>GSHMSDWDPVVKEWLVDTGYCCAGGIANAEDGVVFAAAADDDDGWSKLYKDDHEEDTIGEDGNACGKVSINEASTIKAAVDDGSAPNGVWIGGQKYKVVRPEKGFEYNDCTFDITMCARSKGGAHLI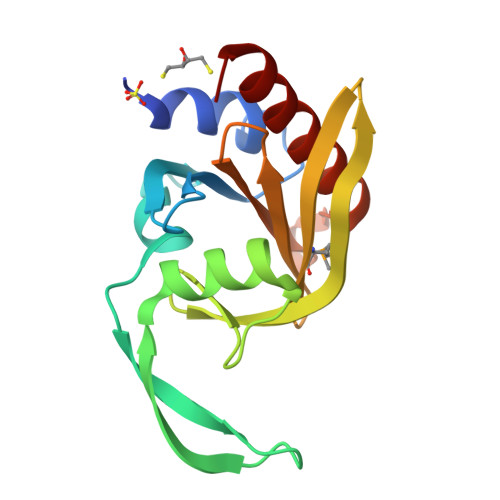KTPNGSIVIALYDEEKEQDKGNSRTSALAFAEYLHQSGY[4x]>GSHMQPMQAMKIERGTILTQPGVFGVFTMFKLRPDWNKVPAMERKGAAEEVKKLIEKHKDNVLVDLYLTRGLETNSDFFFRINAYDLAKAQTFMREFRSTTIGKNADVFETLVGVTKPLNYISKDKSPGLNAGLSSATYSGPAPRYVIVIPVKKNAEWWNMSPEERLKEMEVHTTPTLAYLVNVKRKLYHSTGLDDTDFITYFETDDLTAFNNLMLSLAQVKENKFHVRWGSPTTLGTIHSPEDVIK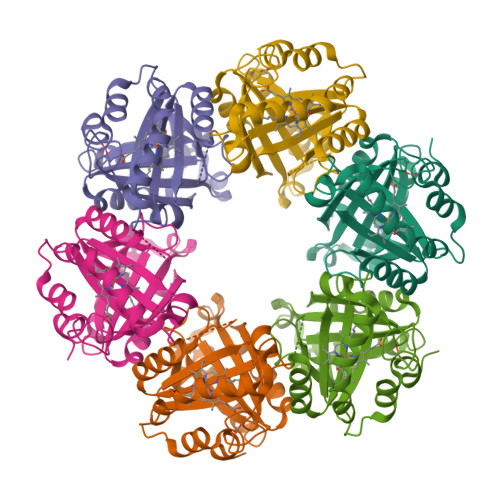ALAD[6x]> SVDFKTYVDQACR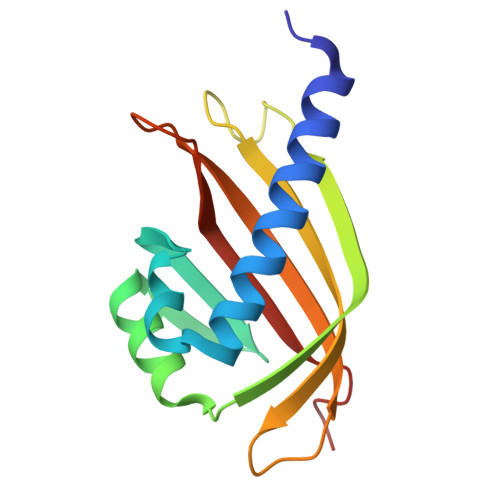AAEEFVNVYYTTMDKRRRLLSRLYMGTATLVWNGNAVSGQESLSEFFEMLPSSEFQISVVDCQPVHDEATPSQTTVLVVICGSVKFEGNKQRDFNQNFILTAQASPSNTVWKIASDCFRFQDWAS> MRGSHHHHHHGSLDFAHPAYSAREQQWMADHPVVKVAVLNLFAPFTLFRTDEQFGGISAAVLQLLQLRTGLDFEIIGVDTVEELIAKLRSGEADMAGALFVNSARESFLSFSRPYVRNGMVIVTRQDPDAPVDADHLDGRTVALVRNSAAIPLLQRRYPQAKVVTADNPSEAMLMVA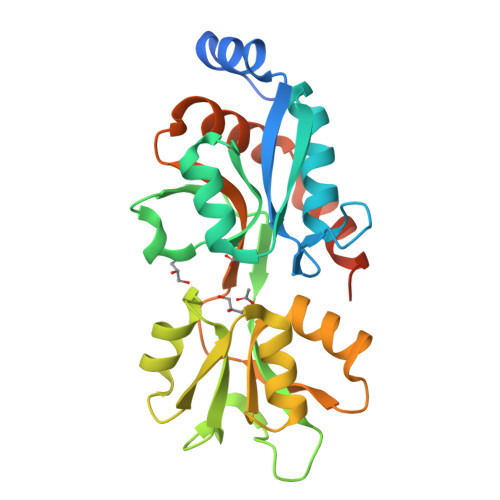NGQADAVVQTQISASYYVNRYFAGKLRIASALDLPPAEIALATTRGQTELMSILNKALYSISNDELASIISRWRGSDGDPRTWYAYRNEI> MDICGELKAENIVEKAINLLSKEDQAGVHFNEISALTRDFCRAILSDLEQSGFTTSELEKEIADKVKIMFAQGYHIEVLQLILEKILDSFISVIREQYHDLQAAASYITTVRD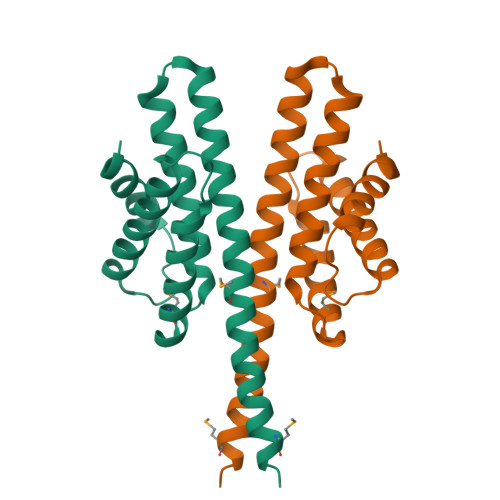HIFKGTSFLLKMALQTQREVIQKQNEALMELST>[2x]MTTQTTPAHIAMFSIAAHGHVNPSLEVIRELVARGHRVTYAIPPVFADKVAATGPRPVLYHSTLPGPDADPEAWGSTLLDNVEPFLNDAIQALPQLADAYADDIPDLVLHDITSYPARVLARRWGVPAVSLSPNLVAWKGYEEEVAEPMWREPRQTERGRAYYARFEAWLKENGITEHPDTFASHPPRSLVLIPKALQPHADRVDEDVYTFVGACQGD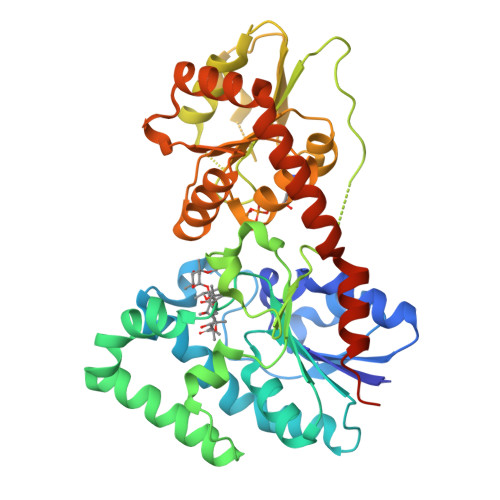RAEEGGWQRPAGAEKVVLVSLGSAFTKQPAFYRECVRAFGNLPGWHLVLQIGRKVTPAELGELPDNVEVHDWVPQLAILRQADLFVTHAGAGGSQEGLATATPMIAVPQAVDQFGNADMLQGLGVARKLATEEATADLLRETALALVDDPEVARRLRRIQAEMAQEGGTRRAADLIEAELPARHERQEPVGDRPNGG>HMDTTHNDTTPQRLMITDMRPLSLETTITSLTRDIITHRFIYLINHECIVRKLDERQATFTFLVNYEMKL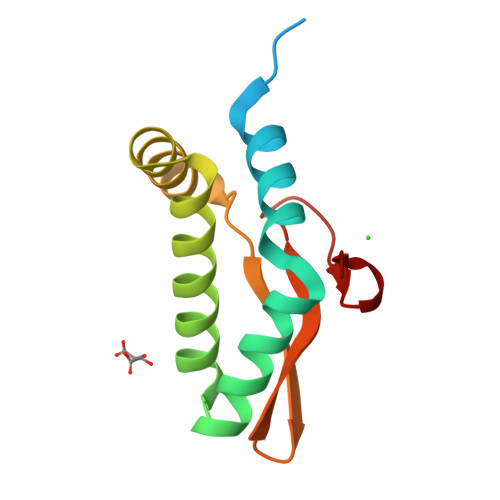LHKVGSTKYKKYTEYNTKYGTFPMPIFINHDGFLECIGIKPTKHTPIIYKYDLNP[3x]>IWLDLKDRIPYYKSDWVDAFNYRVIPSTVDTYFNNLLPAIAFAQDMFDRTDNSYGVNEVLLSSAMAGIVFGVLAGQPLCIVGVTGPISIFNYTVYEIIKPLNTSYFGFMFWICLWSMIFHLLLAFTNVVCLLQYVTTFPCDIFGLFINVVYIQKGIQILTRQFHNTSGEKSVQDGFASVVVALVMTAFGLFFKSFHHYPLFTHKIRTFISDYSTALSVLFWSSFTHFGGYLNDVKFKKLPITKSFFPTSKFNRPQNTWLAYEPIPVKDVFIALPFGIILTILFYFDHNVSSLMAQRHQYKLRKPSSFHYDFALLGLTTCISGVLGIPAPNGLIPQAPLHTETLLVRDSNQN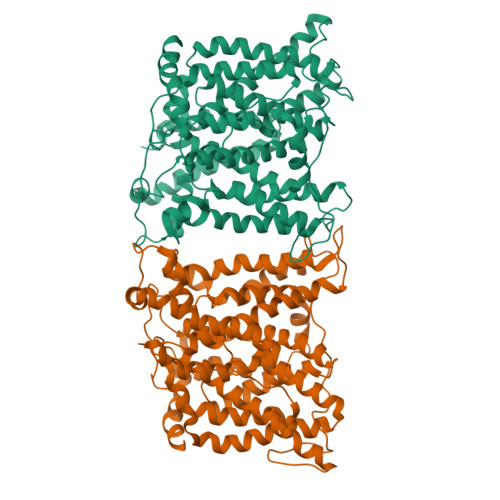VVRCVEQRLTNTFQGLMILGTMTRPLLVCLGEIPQAVLSGLFFIMGINGLMTNVIIHRIVFLFSDPKRRDNNSPLAKISKRSMVIFLCFSLAGFTGEFAITNTIAAIGFPLVLLLSVIVSFSFTY[2x]>XSSDPLVVAASIIGILHLI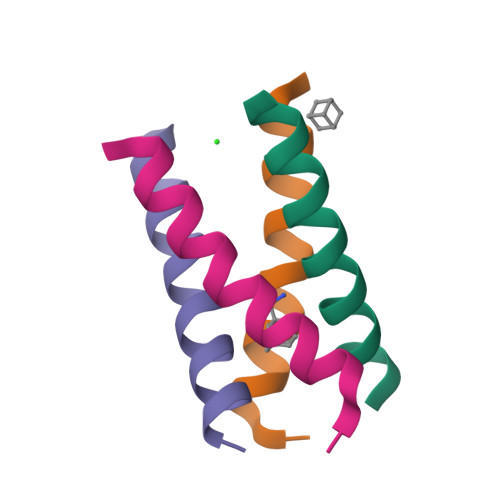LWILDRLX[16x]>MTEAQAIAKQLGGVKPDDEWLQAEIARLKGKSIVPLQQVKTLHDWLDGKRKARKSCRVVGESRTGKTVACDAYRYRHKPQQEAGRPPTVPVVYIRPHQKCGPKDLFKKITEYLKYRVTKGTVSDFRDRTIEVLKGCGVEMLIIDEADRLKPETFADVRDIAEDLGIAVVLVGTDRLDAVIKRDEQVLERFRAHLRFGKLSGEDFKNTVEMWEQMVLKLPVSSNLKSKEMLRILTSATEGYIGRLDEILREAAIRSLSRGLKKIDKAVLQEVAKEYK[7x];>MIEAPDVKPWLFLIKPYEGESL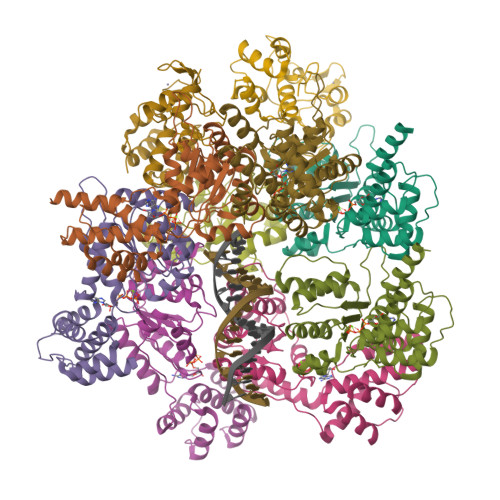SHFLGRFRRANHLSASGLGTLAGIGAIVARWERFHFNPRPSQQELEAIASVVEVDAQRLAQMLPPAGVGMQHEPIRLCGACYAESPCHRIEWQYKSVWKCDRHQLKILAKCPNCQAPFKMPALWEDGCCHRCRMPFAEMAKLQKV[3x]>[2x]GKETGNMPEIKKQPIASAVPDFNADSAYAYVANQVAFGPRVPNTAAHKACGDYLASELKRFGAKVYQQEAILTAYDGTKLEARNIIGSFDPENSKRVLLFAHWDSRPYSDHDPDPSKHRTPLDGADDGGSGVGALLEIARQIGQKAPGIGIDIIFFDAEDYGTPEFVTDYTPDSWCLGTQFWAKNPHVPNYTA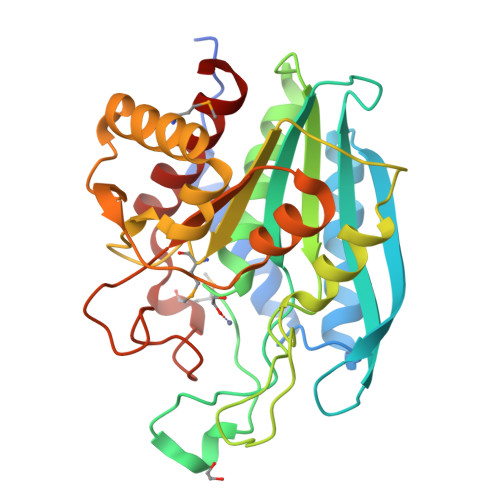EYGILLDMVGGKNATFFKEQQSLRAAAPIVEMVWSAARDLGYGKYFINAAGGAITDDHQYVISGRNIPSIDIINYDPESKTGFASYWHTQKDNMENIDRETLKAAGQTVLEVIYNR1-(3-methyl-1,2,4-thiadiazol-5-yl)-1,4-diazepane | C8 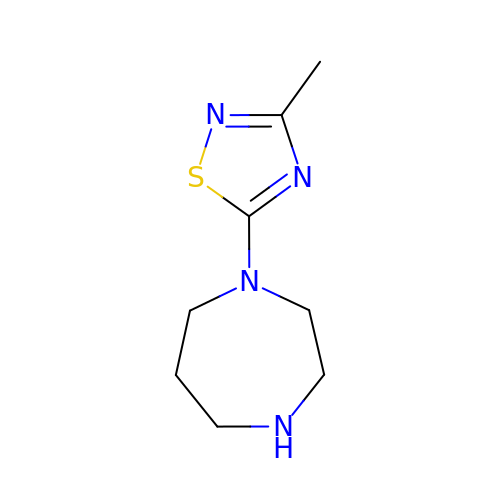H14 N4 S | MZKLTZIEMSVRMI-UHFFFAOYSA-N>MNLPTAQEVQGLMARYIELVDVGDIEAIVQMYADDATVEDPFGQPPIHGREQIAAFFRQGLGGGKVRACLTGPVRASHNGCGAMPFRVEMVWNGQPCA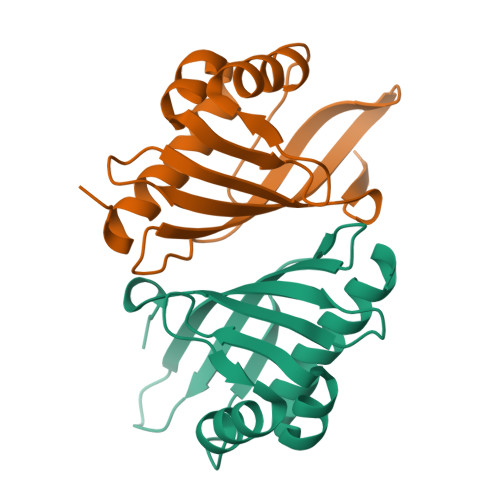LDVILVMRFDEHGRIQTMQAYWSEVNLSVREPQ[2x]NAMPT functions as a homo-dimeric enzyme that catalyzes the rate limiting step in the primary salvage pathway for NAD synthesis, the transfer of a phosphoribosyl residue from 5-phosphoribosyl-1-pyrophosphate (PRPP) to nicotinamide (NAM) to produce nicotinamide mononucleotide (NMN). Crystal structures of NAMPT in numerous ligand-bound forms have been reported. These structures consistently display a NAMPT homo-dimer with two essentially identical active sites at the dimer interface. Typical NAMPT inhibitors were found to occupy the portion of active site responsible for NAM binding and a tunnel-shaped cavity extending from the NAM binding site. Furthermore, we determine the crystal structures of six NAMPT mutants in the apo form and in complex with various inhibitors and present a definitive model to explain the differential effects of the mutations on various structural classes of NAMPT inhibitors.

The RD cell line with the S165F mutation is almost 1000-fold resistant to GNE-618, but only10-fold and 100-fold resistant to APO866 and GMX1778, respectively, demonstrating that inhibitors from distinct classes are differentially affected. Cell lines harboring S165F, S165Y, or G217A are preferentially resistant to GNE-618 compared to GMX1778 and APO866. The identification of resistance mutations in S165 was surprising because this residue does not lie within the drug-binding pocket. However, the part of NAMPT structure that is responsible for inhibitor binding is not affected by the S165 mutations. However, expression of S165F/Y mutant NAMPT allows cell survival in the presence of GNE-618, implying that the mutant NAMPT retains a level of enzymatic activity to support sufficient NAD production for cell survival. However, expression of S165F or S165Y mutant NAMPT proteins in a naïve cell line resulted in decreased sensitivity to GNE-618, indicating that these mutations are sufficient to cause resistance to this NAMPT inhibitor.

>MNPAAEAEFNILLATDSYKVTHYKQYPPNTSKVYSYFECREKKTENSKLRKVKYEETVFYGLQYILNKYLKGKVVTKEKIQEAKDVYKEHFQDDVFNEKGWNYILEKYDGHLPIEIKAVPEGFVIPRGNVLFTVENTDPECYWLTNWIETILVQSWYPITVATNFREQKKILAKYLLETSGNLDGLEYKLHDFGYRGVSSQETAGIGASAHLVNFKGTDTVAGLALIKKYYGTKDPVPGYSVPAAEHSTITAWGKDHEKDAFEHIVTQFSSVPVSVVSDSYDIYNACEKIWGEDLRHLIVSRSTQAPLIIRPDSGNPLDTVLKVLEILGKKFPVTENSKGYKLLPPYLRVIQGDGVDINTLQEIVEGMKQKMWSIENIAFGSGGGLLQKLTRDLLNCSFKCSYVVTNGLGINVFKDPVADPNKRSKKGRLSLHRTPAGNFVTLEEGKGDLEEYGQDLLHTVFKNGKVTKSYSFDEIRKNAQLNIELEAAHHLEHHHHHHHH[2x]Polyglycine hydrolases (PGHs) are secreted fungal proteases that cleave the polyglycine linker of Zea mays ChitA, a defensive chitinase, thus overcoming one mechanism of plant resistance to infection. PGHs are composed of two domains: the N- and C-domains. The N-domain is a novel tertiary fold with an as-yet unknown function that is found across all kingdoms of life. The C-domain shares structural similarities with class C β-lactamases, including a common catalytic nucleophilic serine.

In the present paper, we discuss the structure of one of these polyglycine hydrolases from F. vanettenii. The structure was solved by molecular replacement using a RoseTTAFold model. Fvan-cmp consists of two distinct domains, the N- and C-domains, that are connected by a linker. The Fvan-cmp N-domain (residues 13–262) consists of four loops, five α-helices and 15 β-strands assembled into a distinct tertiary fold. This distinct structure, as shown in Fig. 3, is comprised of five quasi-identical structural repeats consisting of three β-sheets and an α-helix arranged as EHEE with β-strands in an antiparallel assembly. The Fvan-cmp C-domain (residues 271–616) consists of seven α-helices and one antiparallel β-sheet and resembles a β-lactamase fold. Fvan-cmp shares the same nucleophilic serine found within this motif. Fvan-cmp lacks this glycine and instead contains a phenylalanine in the same structural position. We showed that Fvan-cmp retains two of the three conserved β-lactamase motifs and the core active-site αβα fold but lacks the associated activity.

> EFLPNQRRSNVTSHVETYYSVDGATHAEKSKALKADGYRIVSLSSYGSPDSANYAAIWVQEEGPSFEIIHDADEATYNSWLQTWKSRGYVSTQVSATGPAENAVFAGVMENINVANWFQSCELENPWAFSNTTGNVDVVVKGFRMFGTPEERRYCILGHENVGNEQTTIQYSTPSFTVNFASTFEAETTKRFWRPSRLFLSEDHIITPSFADTSVGKWSHAVDLTKAELKEKIETERAKGLYPIDIQGGGSGSSERFTVVFAERTSPKPRQWNVRGEITGFEDNKAAEEEVDSIMRRFMEKNGVRQAQFAVALEGKTIAERSYTWAEDDRAIVEPDDIFLLASVSKMFLHASIDWLVSHDMLNFSTPVYDLLGYKPADSRANDINVQHLLDHSAGYDRSMSGDPSFMFREIAQSLPTKGAKAATLRDVIEYVVAKPLDFTPGDYSAYSNYCPMLLSYVVTNITGVPYLDFLEKNILDGLNVRLYETAASKHTEDRIVQESKNTGQDPVHPQSAKLVPGPHGGDGAVKEECAGTFAMAASASSLAKFIGSHAVWGTGGRVSSNRDGSLSGARAYVESRGTIDWALTLNTREYISETEFDELRWYSLPDFLSAFPIAG> ETGSAQQLNEDLRLHLLLNTSVTCNDGSPAGYYLKESRGSRRWLLFLEGGWYCFNRENCDSRYDTMRRLMSSRDWPRTRTGTGILSSQPEENPYWWNANMVFIPYCSSDVWSGASSKSEKNEYAFMGALIIQEVVRELLGRGLSGAKVLLLAGSAAGGTGVLLNVDRVAEQLEKLGYPAIQVRGLADSGWFLDNKQYRHTDCVDTITCAPTEAIRRGIRYWNGVVPERCRRQFQEGEEWNCFFGYKVYPTLRSPVFVVQWLFDEAQLTVDNVHLTGQPVQEGLRLYIQNLGRELRHTLKDVPASFAPACLSHEIIIRSHWTDVQVKGTSLPRALHCWDRSLHDSHKASKTPLKGCPVHLVDSCPWPHCNPSC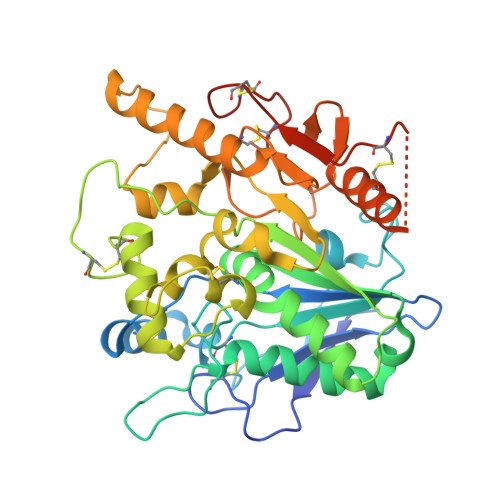PTGTHHHHHHHHHH> MSSEATLDSEFTDYKAMFRYEAKVFKELVDSVSKILDEGLFIITGEGLRLRGMDPARVALVDIEIPSSSFFDFYMAGDVERVELGVNMETLKGVVARAKKGDQLEVRVREDKVLFIVESVVLRRYLLPNLEVIVDVPEDISLEFDATATVIADVVKKTLRDVELVGDIVEFDAGEDYLSIRSVGPERRRVETRLTRESPALIDLEVKEPATSRYDVGYLKRMLGVAKIAESIELSFSTDKPLKMVFKS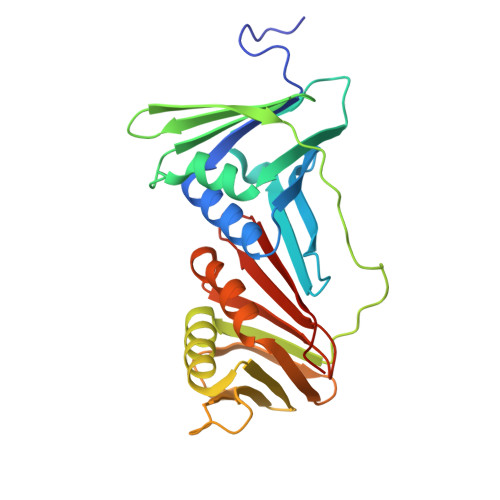PDGSRVTYLLAPSTG methyl 5-{3-[(4S)-6-amino-5-cyano-3-methyl-4-(propan-2-yl)-2,4-dihydropyrano[2,3-c]pyrazol-4-yl]-5-cyanophenyl}thiophene-2-carboxylate 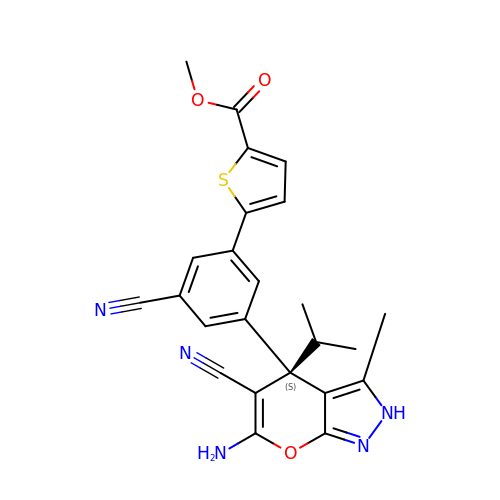| C24 H21 N5 O3 S | CTJJXDPGSNOYMV-DEOSSOPVSA-N The anaerobic, Ni-dependent CODH has a homodimeric structure containing a total of five metalloclusters, called the B-, C-, and D-clusters. The C-cluster is the site of CO/CO2 interconversion and is composed of a [Ni-3Fe-4S] cubane connected through a linking sulfide (SL) to a unique iron site (Feu). Here, we report the crystal structure of the CODH from Desulfovibrio vulgaris (DvCODH), which reveals a surprising and unprecedented conformational rearrangement of metal ions in the C-cluster and provides the first visualization of the cluster in an oxidized state. The overall fold and cluster placement of DvCODH is highly similar to other structurally characterized CODHs.

We next investigated whether this altered C-cluster state is redox dependent. Pre-formed crystals of as-isolated DvCODH (batch 2, containing the altered cluster) were incubated with the reductant sodium dithionite. Strikingly, the resulting crystal structure displays the canonical C-cluster with Ni, Feu, and SL rearranged into their catalytically-relevant positions. Remarkably, oxidation of the reduced C-cluster by exposure to O2 results in reformation of the unusual cluster architecture, whereas both the D- and B-clusters remain intact. Together, these results suggest that this altered cluster is an oxidized form of the C-cluster and that this multi-metal ion rearrangement is reversible. In the present work, the metal migration of C-cluster atoms is more dramatic than in these other examples, with Ni moving ~3 Å and adopting an entirely new coordination environment, and Feu and SL moving ~1.9 and 2.6 Å, respectively, with Feu also taking on a new coordination environment. This C-cluster rearrangement from oxidized to reduced appears to involve what amounts to a ‘molecular cartwheel’ with Ni, Feu, and SL following the same trajectory to end up in their canonical positions.

>[2x]MWSHPAVRKSSSKTIRSRSIWDDAHAMLEKAKAEGISTVWDRAAEQTPACKFCELGTTCRNCIMGPCRIANRKDGKMRLGVCGADADVIVARNFGRFIAGGAAGHSDHGRDLIETLEAVAEGKAPGYTIRDVAKLRRIAAELGVADAATRPAHDVAADLVTICYNDFGSRRNALAFLARAPQVRRDLWQRLGMTPRGVDREIAEMMHRTHMGCDNDHTSLLVHAARTALADGWGGSMIGTELSDILFGTPRPRQSTVNLGVLRKDAVNILVHGHNPVVSEMILAATREPAVRQAAQDAGAADINVAGLCCTGNELLMRQGIPMAGNHLMTELAIVTGAADAIVADYQCIMPSLVQIAACYHTRFVTTSPKGRFTGATHVEVHPHNAQERCREIVMLAIDAYTRRDPARVDIPSQPVSIMSGFSNEAILEALGGTPKPLIDAVVAGQIRGFVGIVGCNNPKIRQDSANVTLTRELIRRDIMVLATGCVTTAAGKAGLLVPEAASKAGEGLAAVCRSLGVPPVLHMGSCVDNSRILQLCALLATTLGVDISDLPVGASSPEWYSEKAAAIAMYAVASGIPTHLGLPPNILGSENVTAMALHGLQDVVGAAFMVEPDPVKAADMLEAHIVARRARLGLTS>MRMIVGHGIDIEELASIESAVTRHEGFAKRVLTALEMERFTSLKGRRQIEYLAGRWSAKEAFSKAMGTGISKLGFQDLEVLNNERGAPYFSQAPFSGKIWLSISHTDQFVTASV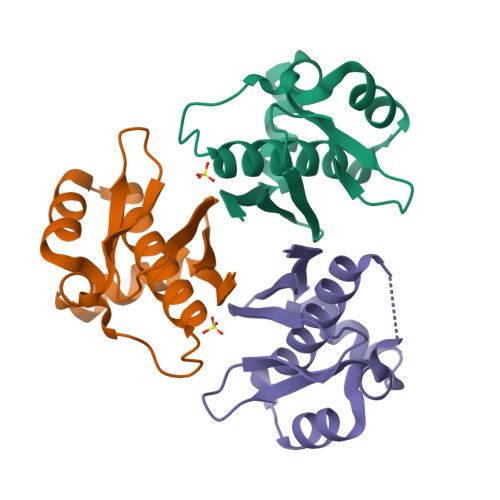ILEENHES[3x]>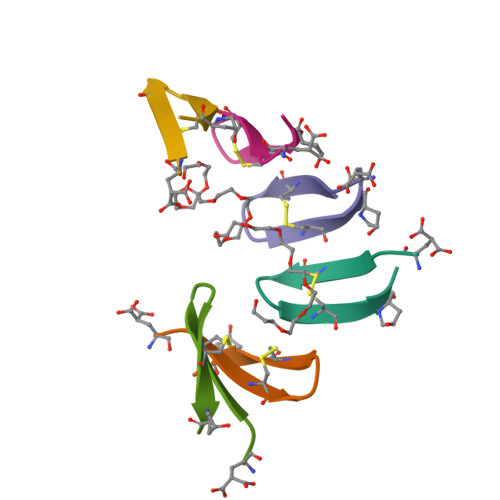EGYKCVWKTCMPA[6x]The NADPH-dependent imine reductase from Ajellomyces dermatitidis (AdRedAm) catalyzes the reductive amination of certain ketones with amine donors supplied in an equimolar ratio. The two AdRedAm monomers associate to form a dimer in which reciprocal domain sharing results in the formation of a large active-site cleft between the N-terminal domain of one monomer and the C-terminal domain of its partner. One of them, AdRedAm from Ajellomyces dermatitidis, has been reported to be more stable than AspRedAm and thus perhaps more suitable for process applications.

The third form, which belongs to space group P3121 and was refined to 1.52 Å resolution, has one molecule (one half-dimer) in the asymmetric unit. This structure was again complexed with NADP+ and also with the substrate 2,2-difluoroacetophenone. In the complex of AdRedAm with 15, the phenyl ring of the substrate is stacked against the side chain of Met176; the carbonyl group of the ketone is coordinated to the phenolic hydroxyl of the side chain of Tyr177 at a distance of 3.0 Å. The F atoms are again positioned 3.2 and 3.3 Å from the O2D atom of the ribose sugar, suggesting again that these inter­actions may be significant in permitting the reduction of the ketone by the cofactor to some extent, but only in the case where F atoms are present. In addition, the ketone 15 presents its re face to the cofactor, which would result in the experimentally observed (S)-alcohol product. The complex illustrates the imperfect binding of the fluorinated ketone 15 for either amine or alcohol production, and also provides a basis for understanding the stereoselectivity of AdRedAm for transformations of substrates in this series.

> MANSPVSVFGLGAMGTALATQFLRKGHKTTVWNRTPAKAQPLIAIGASHAPTIDSAAAASSLLIICQLDKASVMQTLQQAPTAWAAKTIVDLTNGTPAHARETADWALAHGARYIHGGIMAVPFMIGQPDAMILYSGPAEVFEGVKDTLSVLGTNTYVGEDVGLASLHDLALLSGMYGLFSGFTHAVALVQSANIPAAGFVATQLIPWLTAMTQHLNLLATQVDEKDYGDGGSSLDMQAKAAPNILEASQAQGVSVELIQPIFKLIERRVEEGKGSEGLAALVGMIMK>QDKGSVGIAMPTKSSARWIDDGNNIVKQLQEAGYKTDLQYADDDIPNQLSQIENMVTKGVKVLVIASIDGTTLSDVLKQAGEQGIKVIAYDRLIRNSGDVSYYATFDNFQVGVLQATSITDKLGLKDGKGPFNIELFGGSPDDNNAFFFYDGAMSVLKPYIDSGKLVVKSGQMGMDKVGTLRWDPATAQARMDNLLSAYYTDAKVDAVLSPYDGLSIGIISSLKGVGYGTKDQPLPVVSGQDAEVPSVKSIIAGEQYSTIFKDTRELAKVTVNMVNAVMEGK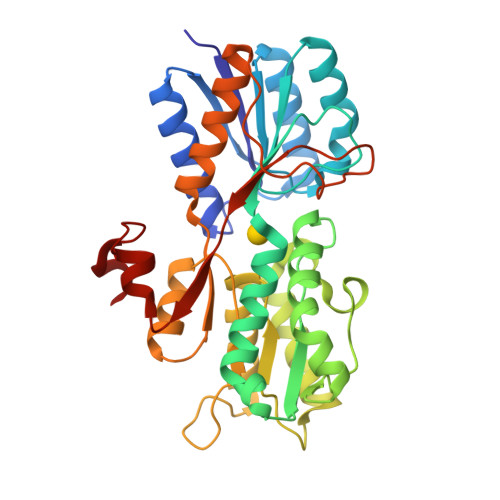EPEVNDTKTYENGVKVVPSYLLKPVAVTKENYKQVLVDGGYYKEDQLK[2x]>[2x]SNAMRVRNRKGATELLEANPQYVVLN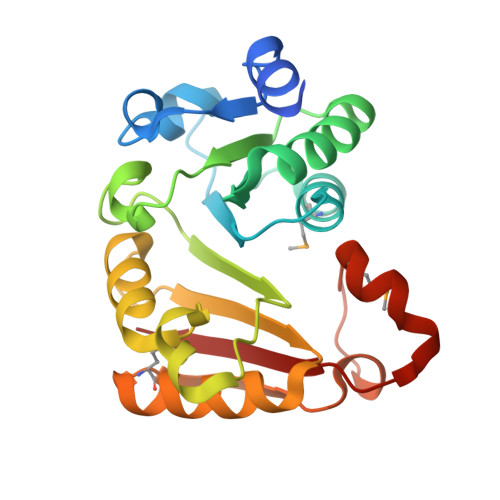PLEAKAKWRDLFGNDNPIHVEVGSGKGAFVSGMAKQNPDINYIGIDIQKSVLSYALDKVLEVGVPNIKLLWVDGSDLTDYFEDGEIDRLYLNFSDPWPKKRHEKRRLTYKTFLDTFKRILPENGEIHFKTDNRGLFEYSLVSFSQYGMKLNGVWLDLHASDFEGNVMTEYEQKFSNKGQVIYRVEAEF>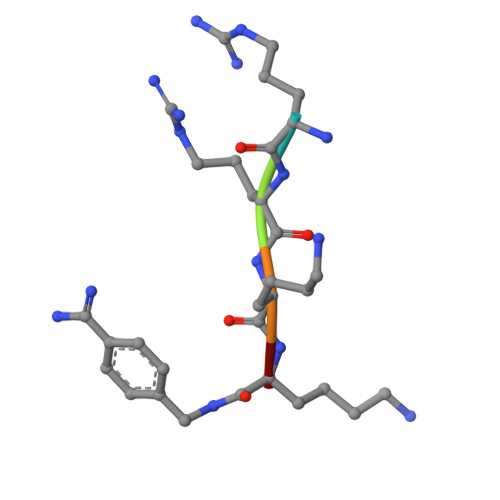 RRKKX> MSATGLEVFDRTLHKTHAWLKAIMEELGTEDRHKAYLALRAVLHALRDRLTVEEVAQLAAQLP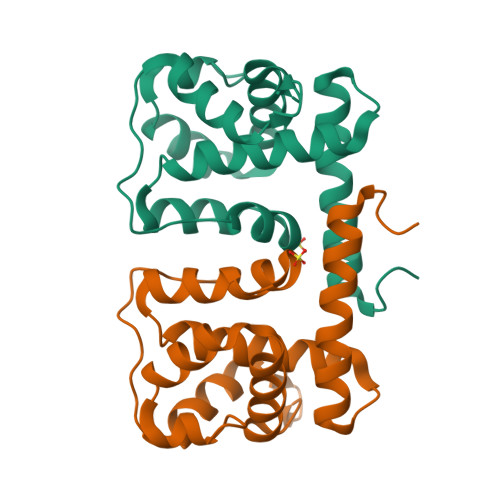MLVRGLYYEGWDPTGKPLKERHKEAFLAHVAEELKTPSGPAVDPEAATRAVFKVLSREISQGELEDVLGLLPKELRALWPQG>[2x]MILVTGSSGQIGTELVPYLAEKYGKKNVIASDIVQRDTGGIKFITLDVSNRDEIDRAVEKYSIDAIFHLAGILSAKGEKDPA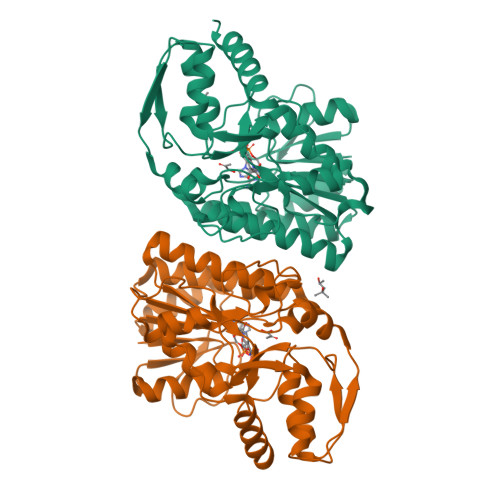LAYKVNMNGTYNILEAAKQHRVEKVVIPSTIGVFGPETPKNKVPSITITRPRTMYGVTKIAAELLGQYYYEKFGLDVRSLRYPGIISYKAEPTAGTTDYAVEIFYYAVKREKYKCYLAPNRALPMMYMPDALKALVDLYEADRDKLVLRNGYNVTAYTFTPSELYSKIKERIPEFEIEYKEDFRDKIAATWPESLDSSEASNEWGFSIEYDLDRTIDDMIDHISEKLGIEGKHAL>MGRRRSHERRDLPPNLYIRNNGYYCYRDPRTGKEFGLGRDRRIA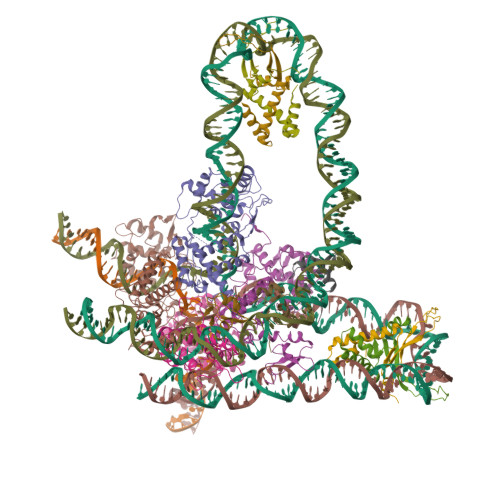ITEAIQANIELFSGHKHKPLTARINSDNSVTLHSWLDRYEKILASRGIKQKTLINYMSKIKAIRRGLPDAPLEDITTKEIAAMLNGYIDEGKAASAKLIRSTLSDAFREAIAEGHITTNHVAATRAAKSEVRRSRLTADEYLKIYQAAESSPCWLRLAMELAVVTGQRVGDLCEMKWSDIVDGYLYVEQSKTGVKIAIPTALHIDALGISMKETLDKCKEILGGETIIASTRREPLSSGTVSRYFMRARKASGLSFEGDPPTFHELRSLSARLYEKQISDKFAQHLLGHKSDTMASQYRDDRGREWDKIEIK[4x];>ALTKAEMSEYLFDKLGLSKRDAKELVELFFEEIRRALENGEQVKLSGFGNFDLRDKNQRPGRNPKTGEDIPITARRVVTFRPGQKLKSRVENASPK[2x];>[2x]MTKSELIERLATQQSHIPAKTVEDAVKEMLEHMASTLAQGERIEIRGFGSFSLHYRAPRTGRNPKTGDKVELEGKYVPHFKPGKELRDRANIYG;>[3x]MYLTLQEWNARQRRPRSLETVRRWVRESRIFPPPVKDGREYLFHESAVKVDLNRP>[2x]DHQVKDSLEQLRCHFTWELSIDDDEMPDLENRVLDQIEFLDTKYSVGIHNLLAYVKHLKGQNEEALKSLKEAENLMQEEHDNQANVRSLVTW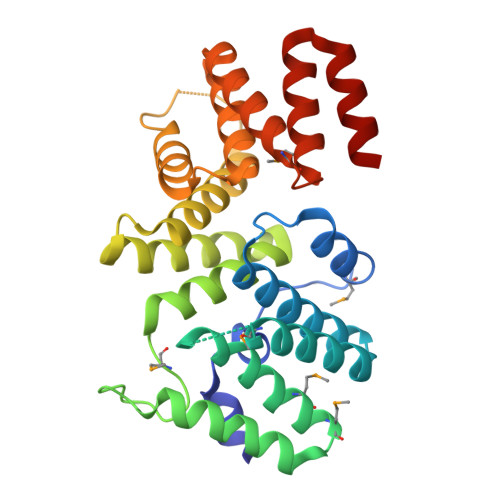GNFAWMYYHMGRLAEAQTYLDKVENICKKLSNPFRYRMECPEIDCEEGWALLKCGGKNYERAKACFEKVLEVDPENPESSAGYAISAYRLDGFKLATKNHKPFSLLPLRQAVRLNPDNGYIKVLLALKLQDEGQEAEGEKYIEEALANMSSQTYVFRYAAKFYRRKGSVDKALELLKKALQ> GKMLVVYMTLGYPNVQSFKDFII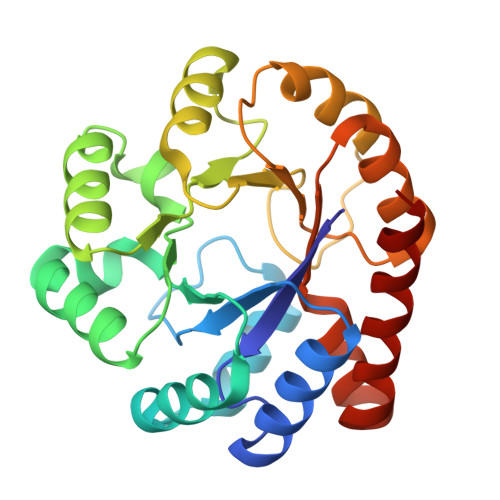GAVENGADILELGIPPKYAKYDGPVIRKSYDKVKGLDIWPLIEDIRKDVGVPIIALTYLEDWVDQLENFLNMIKDVKLDGILFPDLLIDYIDDLDKIDGIIKNKGLKNVIFTSPSVPDLLIHKVSKISDLFLYYGVRPTTGVPIPVSVKQLINRVRNLVENKLIVGFGLSSESDLRDALSAGADGIAIGTVFIEEIERNGVKSAINLVKKFRAILDEY> GPGSNCGPPPTLSFAAPMDITLTETRFKTGTTMKYTCLPGYVRSHSTQTMTCNSDGEWVYNTFCIYKRCRHPGE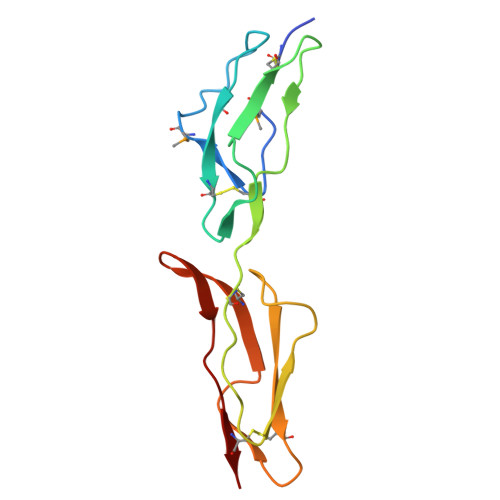LRNGQVEIKTDLSFGSQIEFSCSEGFFLIGSTTSRCEVQDRGVGWSHPLPQCEI>DIISVALKRHSTKAFDASKKLTAEEAEKIKTLLQYSPSSTNSQPWHFIVASTEEGKARVAKSAAGTYVFNERKMLDASHVVVFCAKTAMDDAWLERVVDQEEADGRFNTPEAKAANHKGRTYFADMHRVDLKDDDQWMAKQVYLNVGNFLLGVGAMGLDAVPIEGFDAAILDEEFGLKEKGFTSLVVVPVGHHSVEDFNATLPK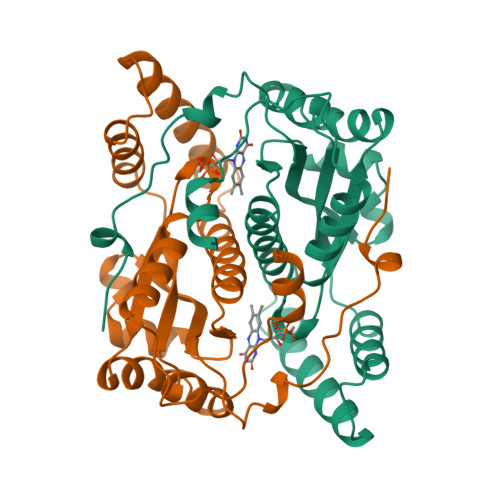SRLPLSTIVTEC[4x]R388 has 35 genes assorted in functional groups or modules, among them, a gene coding for an antirestriction protein called ArdC. Interestingly, ArdC contains an N-terminal ssDNA binding domain and a C-terminal metalloprotease domain. ArdC is structurally similar to DNA-binding dependent metalloproteases involved in the maintenance of genetic stability such as Spartan or IrrE. In summary, our results indicate a new mechanism of DNA antirestriction played by protein ArdC, by which plasmids increase their conjugation host range.

R388 ArdC crystal structure was solved at 2.6 Å resolution using a selenomethionine-derivative protein structure solved by single anomalous dispersion as described in Materials and Methods. Using this preliminary structure, the apo ArdC structure was solved at 2.0 Å resolution by molecular replacement (MR). Apo ArdC crystallized in the H3 space group containing one molecule per asymmetric unit. ArdC is composed of two structural domains: An N-terminal domain (residues 1–134) and a C-terminal domain (residues 151–297) joined by a long and flexible loop (135–150). Electron density was not observed for the N-terminal residues 1–6, the flexible small loop residues 33–39, residues 136–141 in the region connecting both domains and C-terminal residues 294–297. The N-terminal domain is composed of three α-helices (α1-α3), a three-stranded β-sheet (β1, β3, and β4) that supports a long and protuberant β-hairpin (β3-β4), a smaller two-stranded antiparallel β-sheet formed by β2 and β5, as well as three 310 helices labeled from η1 to η3. The C-terminal domain is composed of six α-helices (α4-α9) and short three-stranded antiparallel β-sheets (β6-β8) as shown in Fig 2A and 2B. The surface electrostatic map reveals a positively charged groove in the region of the N-terminal domain adjacent to the C-terminal domain, suggesting a DNA binding site between both structural domains. The surface electrostatic map revealed a negatively charged catalytic pocket. IrrE protects D. radiodurans from UV radiation DNA damage by proteolysis of a negative transcriptional regulator, DdrO, which represses the expression of DNA damage response genes involved in SOS response. These proteins belong to the gluzinzin metalloprotease family characterized by the presence of the conserved residues HExxH located on the “active site helix” (α5 in ArdC) and an additional conserved motif (E,H)xx(A,F,T,S,G) located in the contiguous α-helix or “glutamate helix” (α7 in ArdC).

> MNAKTKFDLYQHVTDRIIASIEAGTPAWRKPWTGEAATMQMPLRSNGEAYRGINVVMLWLTAAEKGYRSAYWFTYRQAKELGGQVRKGEKGSTVVKFGTIEREDEQTGEEKKIPYLKGYTVFNADQIDGLPEQYHAAPAEAARDLGTAADPELDAFFAATGADIRTSSEPRAYYNPTGDYIHMPPIATFHSAAGYYATLAHEATHWTGHKSRLDRFSRFSDRKSYAFEELIAEIGNCMLCASLGLIPDFDQSAAYVQSWLRALKDDKRLIFKAATEAQKAADLLQENAANFQRKEAA> EEVLLDTTGETSEIGWLTYPPGGWDEVSVLDDQRRLTRTFEACHVAGAPPGTGQDNWLQTHFVERRGAQRAHIRLHFSVRACSSLGVSGGTCRETFTLYYRQAEEPDSPDSVSSWHLKRWTKVDTIAADESFPSSSSSSSSSSSSAAWAVGPHGAGQRAGLQLNVKERSFGPLTQRGFYVAFQDTGACLALVAVRLFSYTCPAVLRSFASFPETQASGAGGASLVAAVGTCVAHAEPEEDGVGGQAGGSPPRLHCNGEGKWMVAVGGCRCQPGYQPARGDKACQACPRGLYKASAGNAPCSPCPARSHAPNPAAPVCPCLEGFYRASSDPPEAPCTGPPSAPQE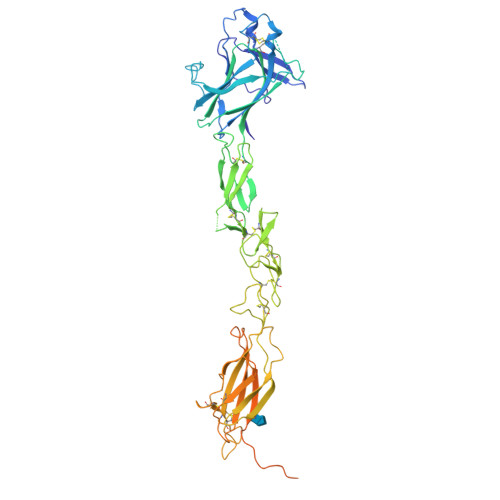LWFEVQGSALMLHWRLPRELGGRGDLLFNVVCKECEGRQEPASGGGGTCHRCRDEVHFDPRQRGLTESRVLVGGLRAHVPYILEVQAVNGVSELSPDPPQAAAINVSTSHEVPSAVPVVHQVSRASNSITVSWPQPDQTNGNILDYQLRYYDQAEDESHSFTLTSETNTATVTQLSPGHIYGFQVRARTAAGHGPYGGKVYFQ>[2x]SGSAEIGTGFPFDP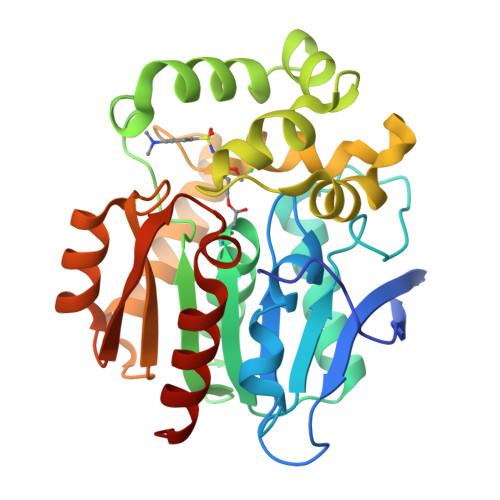HYVEVLGERMHYVDVGPRDGTPVLFLHGNPTSSYVWRNIIPHVAPTHRCIAPDLIGMGKSDKPDLGYFFDDHVRFMDAFIEALGLEEVVLVIHDWGSALGFHWAKRNPERVKGIAFMEFIRPIPTWDEWPEFARETFQAFRTTDVGRKLIIDQNVFIEGTLPCGVVRPLTEVEMDHYREPFLNPVDREPLWRFPNELPIAGEPANIVALVEEYMDWLHQSPVPKLLFWGTPGVLIPPAEAARLAKSLPNCKAVDIGPGLNLLQEDNPDLIGSEIARWLSTLEISG> GSSMASANLEGDALHTLRVTLVDPNNVLQSWDPTLVNPCTWFHVTCNNENSVIRVDLGNAELSGHLVPELGVLKNLQYLELYSNNITGPIPSNLGNLTNLVSLDLYLNSFSGPIPESLGKLSKLRFLRLNNNSLTGSIPMSLTNITTLQVLDLSNNRLSGSVPDNGSFSL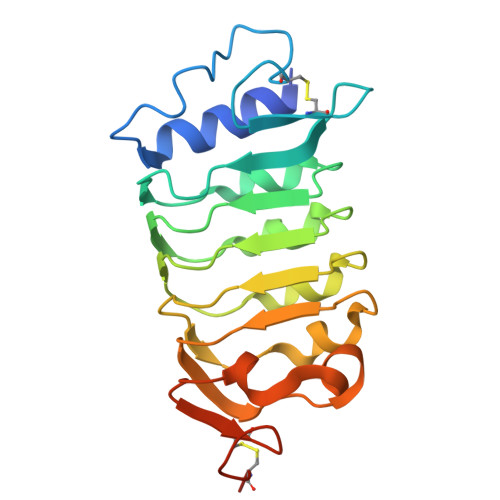FTPISFANNLDLCGPVTSHPCPLEGSLENLYFQ>GPMGSAQLLKSVFVKNVGWATQLTSGAVWVQFNDGSQLVVQAGVSSISYTSPNGQTT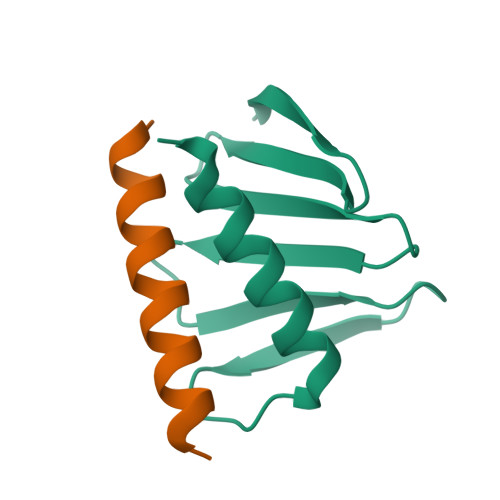RYGENEKLPDYIKQKLQCLSSILLMFSNPTPNFH[3x];>[3x]GGSLTEQDRQLRLLQAQIQRLLEAQSLM>MADKIKVSLLGSTGMVGQKMVKMLAKHPYLELVKVSASPSKIGKKYKDAVKWIEQGDIPEEVQDLPIVSTNYEDHKDVDVVLSALPNELAESIELELVKNGKIVVSNASPFRMDPDVPLINPEINWEHLELLKFQKERKGWKGILVKNPNCTAAIMSMPIKPLIEIATKSKIIITTLQAVSGAGYNGISFMAIEGNIIPYIKGEEDKIAKELTKLNGKLENNQIIPANLDSTVTSIRVPTRVGHMGVINIVTNERINIEEIKKTLKNFKSLPQQKNLPTAPKQPIIVRDEEDRPQPIIDVNAESGMAVTVGRIRHENNVLRLVVLGDNLVRGAA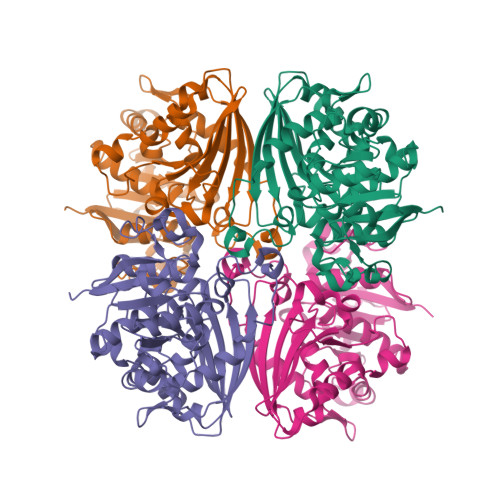GITILTVEVMKELGYI[4x]Epstein–Barr virus (EBV), a member of the Gammaherpesviridae, encodes the Bcl-2 homolog BHRF1, a potent inhibitor of Bcl-2-mediated apoptosis. EBV BHRF1 is a Bcl-2 homolog that potently inhibits host intrinsic apoptosis via direct inactivation of cellular proapoptotic Bcl-2 proteins Bak and Bim and selectively interacts with a subset of proapoptotic proteins (Bid, Puma, and Bax) to regulate apoptosis. Despite sharing very weak sequence identity with its cellular counterparts Bcl-2 (21.7%), Bcl-xL (17.9%), Bcl-w (18.4%), Mcl-1 (9.6%), Bfl-1/A1 (17.8%), and Bcl-B (21.5%), BHRF1 adopts the conserved alpha helical Bcl-2 fold comprising eight α-helices, with helices α2–α5 forming the canonical hydrophobic ligand-binding groove which provides the interaction site for the BH3-motif peptide. BHRF1 engages BH3 peptides using the canonical ligand-binding groove of its Bcl-2 fold and maintains a salt bridge between an Arg residue with a conserved Asp residue in the BH3 motif mimicking the canonical ionic interaction seen in host Bcl-2:BH3 motif complexes.

The structure of the BHRF1–BidBH3 complex was refined to a resolution of 2.78 Å, whereas the BHRF1–Puma BH3 complex was refined to 2.0 Å resolution. The BHRF1–Puma BH3 complex showed a clear and continuous electron density map for BHRF1 residues 2–94 and 96–156, as well as Puma BH3 motif peptide residues 131–151. Similar to the BHRF1–Bid BH3 complex, BHRF1–Puma BH3 adopted a globular monomeric topology. The four conserved hydrophobic residues of the Puma BH3 motif, I137, L141 M144, and L148, protrude into four hydrophobic pockets in the canonical ligand-binding groove, with an additional hydrophobic pocket occupied by a fifth hydrophobic residue W133. Furthermore, a conserved ionic interaction was also found in the BHRF1–Puma BH3 complex between R100BHRF1 and D146Puma. These salt bridges were supplemented by additional hydrogen bonds between the carboxyl group of E89BHRF1 and the NδH side-chain group of R135Puma, and between the G99BHRF1 main-chain amide group and the side-chain carboxyl and amide group of N149Puma. The fifth hydrophobic pocket of BHRF1 is utilized by Puma BH3, where the structurally equivalent residue to Bid I83 is A134 or W133. The binding mode for Bcl-xL–Puma BH3 differs from that of the BHRF1 complex. A similar trend can be observed in BHRF1–Puma BH3 and KsBcl-2–Puma BH3 complexes, where BHRF1 shows nearly threefold reduced affinity for Puma BH3. The F72W BHRF1(1–160) AlphaFold model superimposition with the experimentally determined structure of BHRF1–PumaBH3 resulted in an RMSD value of 0.48 Å, confirming that the AlphaFold-generated structure was nearly identical to the experimental structures over the backbone atoms.

> MGSHHHHHHSQDPMAYSTREILLALCIRDSRVHGNGTLHPVLELAARETPLRLSPEDTVVLRYHVLLEEIIERNSETFTETWNRFITHTEHVDLDFNSVFLEIFHRGDPSLGRALAWMAWCMHACRTLCCNQSTPYYVVDLSVRGMLEASEGLDGWIHQQGGWSTLIEDNIPG;> EEQWAREIGAQLRRMADDLNAQYERR>[2x]GAMGSEKSPSAQELKEQGNRLFVGRKYPEAAACYGRAITRNPLVAVYYTNRA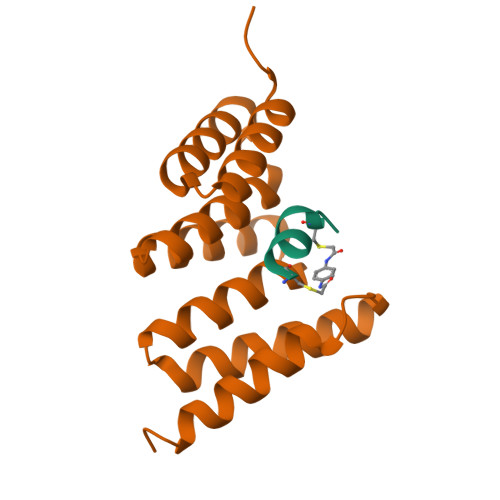LCYLKMQQHEQALADCRRALELDGQSVKAHFFLGQCQLEMESYDEAIANLQRAYSLAKEQRLNFGDDIPSALRIAKKKRWNSIEERR;>[2x]XCWEAWLLCETX>[6x]MSSFSTQTPYPNLAVPFFTSIPNGLYPSKSIVISGVVLSDAKRFQINLRCGGDIAFHLNPRFDENAVVRNTQINNSWGPEERSLPGSMPFSRGQRFSVWILCEGHCFKVAVDGQHICEYSHRLMNLPDINTLEVAGDIQLTHVET

Galectins are multi-purpose effectors acting via interactions with distinct counterreceptors based on protein-glycan/protein recognition. We report here the first crystallographic information on the N-terminal extension of the carbohydrate recognition domain of rat galectin-5, which is precisely described as an N-tailed proto-type-like galectin. The overall fold in ligand-free and -loaded rGal-5 is composed of two antiparallel β-sheets (F1 to F5 and S1 to S6 strands) that form the characteristic β-sandwich structure. The presented data shows that the N-terminal extension can adopt an ordered structure and shapes the hypothesis that a ligand-induced shift in the equilibrium between flexible and ordered conformers potentially acts as a molecular switch, enabling new contacts in this region.

Ligand-free full-length rGal-5 crystallizes in the monoclinic P21 space group and diffracts to a resolution of 1.7 Å. The core of the different protein units can readily be superimposed onto each other, as revealed by the low average root mean square deviation (RMSD) value among them of 0.26 Å for all Cα atoms. Differences are attributed mainly to the N-terminus, and the six protein monomers can be divided into two groups, based on the experimental electron density. In the first group (chains A–C), the 11 residues at the N-terminus are not visible in the electron density map. When inspecting the second group (chains D–F), the electron density for this peptide stretch was clearly observed: the three amino acids from Ser2 to Ser5 form an extra β-strand, named F0, running in antiparallel direction to the C-terminal F1 strand. Residues Thr6 to Asn12 are in a loop, placed in parallel to the axis of the β-sandwich and protruding more than 10 Å from the S1 and F0 strands. The conformation within this loop is stabilized by interactions with symmetry-related molecules: hydrogen bonds between Pro9–His142, Tyr10–Glu103 and Asn12–Gly52 as well as a water bridge between Asn12 and Asn74. In the ligand-free structure, a network of water molecules or the presence of a single glycerol molecule takes the place of the core of a cognate glycan in the preformed contact site. As observed in the hGal-9N structure, a short β-strand is formed in the ligand-free rGal-5.>[2x]MQQLEEALKQLAQGSGSSQALTQVRRWDSACQKLPDANLALISVAGEYAAELANQALDRNLNVMMFSDNVTLEDEIQLKTRAREKGLLVMGPDCGTSMIAGTP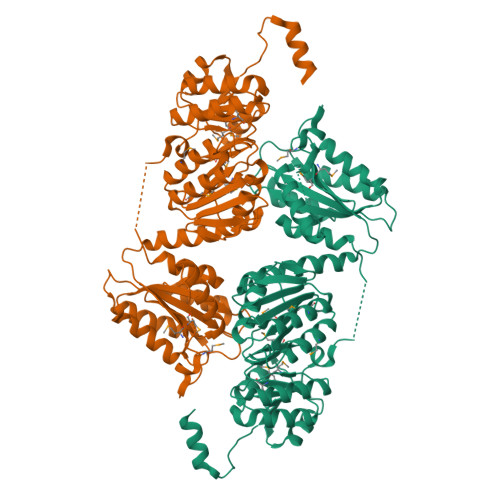LAFANVMPEGNIGVIGASGTGIQELCSQIALAGEGITHAIGLGGRDLSREVGGISALTALEMLSADEKSEVLAFVSKPPAEAVRLKIVNAMKATGKPTVALFLGYTPAVARDENVWFASSLDEAARLACLLSRVTARRNAIAPVSSGFICGLYTGGTLAAEAAGLLAGHLGVEADDTHQHGMMLDADSHQIIDLGDDFYTVGRPHPMIDPTLRNQLIADLGAKPQVRVLLLDVVIGFGATADPAASLVSAWQKACAARLDNQPLYAIATVTGTERDPQCRSQQIATLEDAGIAVVSSLPEATLLAAALIHPLSPAAQQHTPSLLENVAVINIGLRSFALELQSASKPVVHYQWSPVAGGNKKLARLLERLQGHPHHH The manganese transport regulator (MntR) functions as a homodimer and is activated by Mn2+ to repress the expression of two manganese uptake systems, MntABCD and MntH, in response to elevated concentrations of Mn2+. The MntR homologue (BH2807, BhMntR) in Bacillus halodurans is a protein consisting of 139 amino acids, and has 78% sequence identity with MntR from B.subtilis (BsMntR). Each BhMntR subunit was composed of seven α-helices and two β-strands, which could be divided into an N-terminal Helix-Turn-Helix (HTH) DNA binding domain (domain1, residues 1–71) and a C-terminal dimerization domain (domain2, residues 72–139). To further understand the metal binding site of the MntR protein, we determined crystal structures of the apo and manganese-bound forms of MntR from B. halodurans.

The structure was refined to crystallographic Rwork and Rfree values of 18.9% and 22.9%, respectively with good geometry. The C-terminal region of chains A (residue 139) and B (residues 136–139) were poorly ordered, due to lack of electron-density maps. There were few structural differences between apo and Mn2+-bound dimeric forms, with a r.m.s.d. value of 0.49 Å for 276 Cα atoms. When measured between the Cα atoms of Lys41, at the center of helix α3, the domain separation of apo and manganese bound BhMntR are 37.4 Å and 37.5 Å, respectively, while the distance between the Lys41 in apo, Mn2+-bound, and Zn2+-bound BsMntR are 39.2 Å, 32.1Å and 30.7Å, respectively. There was little domain movement between apo and Mn2+-bound BhMntR, possibly due to crystal packing or the presence of positively charged ions of Na+ (~0.5 M) and Mg2+ (~0.4 M) during the crystallization process.

>[2x]MPTPSMEDYLERIYLLIEEKGYARVSDIAEALEVHPSSVTKMVQKLDKSDYLVYERYRGLILTAKGKKIGKRLVYRHDLLEDFLKMIGVDSDHIYEDVEGIEHHLSWDAIDRIGDLVQYFQEDPSRLNDLREVQKKNEE>[8x]MKEIKLILTDIDGV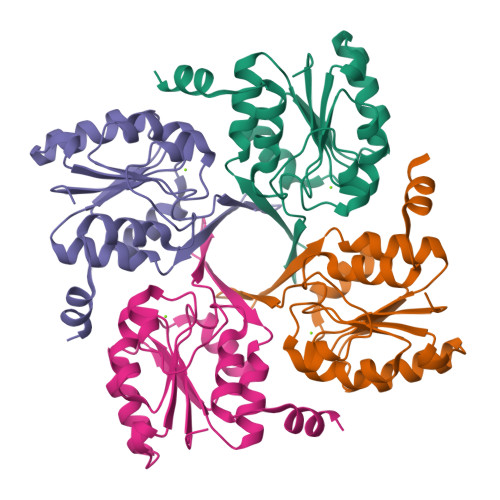WTDGGMFYDQTGNEWKKFNTSDSAGIFWAHNKGIPVGILTGAKTEIVRRRAEKLKVDYLFQGVVDKLSAAEELCNELGINLEQVAYIGDDLNDAKLLKRVGIAGVPASAPFYIRRLSTIFLEKRGGEGVFREFVEKVLGINLEDFIAVIQ>[18x]ASLAADTPTACCFSYTSRQIPQNFIAAYFETSSQC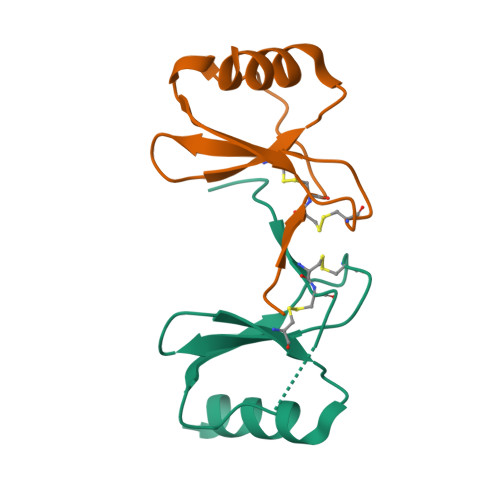SKPGVIFLTKRSRQVCADPSEEWVQKYVSDLELSA The armadillo repeat serves as a scaffold for the development of modular peptide-recognition modules. In order to develop such a system, three crystal structures of designed armadillo-repeat proteins with third-generation N-caps (YIII-type), four or five internal repeats (M-type) and second-generation C-caps (AII-type) were determined at 1.8 Å (His-YIIIM4AII), 2.0 Å (His-YIIIM5AII) and 1.95 Å (YIIIM5AII) resolution and compared with those of variants with third-generation C-caps. All constructs are full consensus designs in which the internal repeats have exactly the same sequence, and hence identical conformations of the internal repeats are expected.

The structure of YIIIM5AII without His tag was determined in the absence of calcium ions and refined at 1.95 Å resolution. This structure is most similar to chains C/D of His-YIIIM5AII (r.m.s.d.s of 1.14 and 0.60 Å for Cα atoms of residues 14–288 of chains A/B and C/D, respectively). A superposition of YIIIM5AII on His-YIIIM5AII based on the N-cap and internal repeats M1–M3 (residues 14–168) reveals that this part is very similar in all chains. However, in this superposition the C-terminal repeats of YIIIM5AII match nicely with the C-terminal repeats of His-YIIIM5AII chains C/D, but they are shifted towards M3 in chains A/B (1.4 Å shift of Trp201 CA towards Leu158 CA). However, in YIIIM5AII the spread between Trp33 Cα-atom distances is extremely large, with the largest distance observed between repeats M3 and M4 (the distances between Trp159 CA and Trp201 CA are 9.42 Å in chain A and 9.43 Å in chain B). This distance is probably too large for binding the target peptide in the desired conformation and this mismatch is located almost at the centre of the putative peptide-binding site. Although YIIIM5AII is considered to be a full consensus design regarding the sequence of internal repeats, the internal repeats are not identical in terms of structure. In the more stable YIIIM5AII structure the side chains of Leu16, Leu20 and Val7 adopt a uniform distribution of side-chain rotamers in all repeats.

>[2x]GPGSELPQMVQQLNSPDQQELQSALRKLSQIASGGDEQIQAVIDAGALPALVQLLSSPNEQILQEALWTLGNIASGGDEQIQAVIDAGALPALVQLLSSPNEQILQEALWTLGNIASGGDEQIQAVIDAGALPALVQLLSSPNEQILQEALWTLGNIASGGDEQIQAVIDAGALPALVQLLSSPNEQILQEALWTLGNIASGGDEQIQAVIDAGALPALVQLLSSPNEQILQEALWTLGNIASGGNEQKQAVKEAGALEKLEQLQSHENEKIQKEAQEALEKLQSH>GDAPAVISDFIYQGASLHNQTDRTGETALHLAARYSRSDAAKRLLEASAD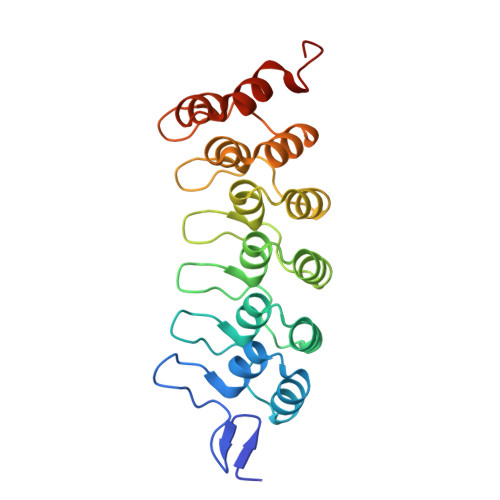ANIQDNMGRTPLHAAVSADAQGVFQILIRNRATDLDARMHDGTTPLILAARLAVEGMLEDLINSHADVNAVDDLGKSALHWAAAVNNVDAAVVLLKNGANKDMQNNREETPLFLAAREGSYETAKVLLDHFANRDITDHMDRLPRDIAQERMHHDIVRLLDEYNLVRSPQLHG[2x]Cellular retinol-binding protein 1 (CRBP1) is the primary transporter of all-trans-retinol (atROL) in the eye, and its inhibition has recently been shown to protect mouse retinas from light-induced retinal damage. We determine binding affinities for the newly identified compounds and elucidate mechanisms of their interaction with the protein by solving high-resolution X-ray structures of human CRBP1 in complex with selected inhibitors. Consistent with the fluorescence data, all of the crystallized compounds acted as competitive inhibitors of CRBP1, occupying the same binding site as atROL. Apart from specific hydrogen bonds, effective binding of retinoids or other high-affinity ligands to CRBPs requires interactions with the entry portal region of the protein, comprising α-helix I and II, as well as hairpin turns between β-strands 3–4 and 5–6.

Three of the newly identified inhibitors of CRBP1 are structurally related by containing a 1,2,4-oxadiazol ring (inhibitors 1–3). The common feature of these compounds is the substitution of the oxadiazol ring at position 3 with a bulky moiety such as 4-methylphenyl cyclopentyl (inhibitors 1 and 2) or diphenylmethyl (inhibitor 3). Position 5 of the oxadiazole ring is coupled to either a thiophene ring (inhibitors 1), a pyrazole ring (inhibitor 2), or a methoxymethylpiperidine moiety present in inhibitor 3. In inhibitor 2, an alternative hydrogen bond is observed between the oxygen atom of the oxadiazole ring and two ordered water molecules. Interestingly, the presence of an N-ethyl group in inhibitor 2, induces an alternative conformation of this molecule in the binding site, which no longer supports hydrogen bonding of the tertiary amine group. Another characteristic interaction site is observed for inhibitors 2 and 6, involving the N(2) nitrogen of their pyrazole rings. In ligand 2, a hydrogen bond is formed between N(2) and an ordered water molecule, which is further stabilized by its interactions with the side chain of T53. The spatial position of these compounds reveals an overlap between the orientation of the β-ionone ring of atROL and the methylphenyl or cyclopentyl rings (inhibitors 1, 2, and 6), diphenylmethyl rings (inhibitors 3 and 5), or the tetrahydronaphthalene moiety of inhibitor 4. The stability of the main chain in the α-helices I/II and the loop between β-strands 5 and 6 correlates with the binding affinity of the tested compounds, showing a notable reduction for ligands with lower binding affinities. It is noteworthy that inhibitor 2, 3, and 5 exhibit a greater propensity to stabilize the α-helices I/II region in comparison to compounds 1, 4, and 6. Additionally, it is interesting to note that certain nonretinoid ligands have the potential to enhance conformational flexibility in segments of CRBP1 that remain well-structured even in the protein’s apo form.

> MPVDFTGYWKMLVNENFEEYLRALDVNVALRKIANLLKPDKEIVQDGDHMIIRTLSTFRNYIMDFQVGKEFEEDLTGIDDRKCMTTVSWDGDKLQCVQKGEKEGRGWTQWIEGDELHLEMRVEGVVCKQVFKKVQHHHHHH> MSTSTVPPDGGEKVVVVGGNDWHEVVAAARAGAAAQAGERIVVNMGPQHPSTHGVLRLILEIEGEIITEARCGIGYLHTGIEKNLEYRNWTQGVTFVTRMDYL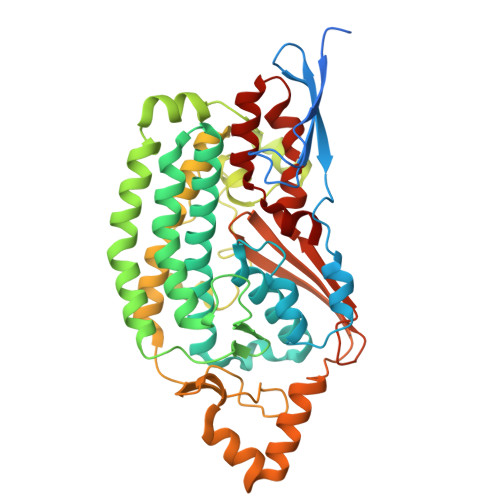SPFFNETAYCLGVEKLLGITDDIPERASVIRVMLMELNRISSHLVALATGGMELGAMSAMFYGFREREEILRVFESITGLRMNHAYIRPGGLAADLPDDAITQVRRLVEILPKRLKDLEDLLNENYIWKARTVGVGYLDLTGCMALGITGPILRSTGLPHDLRKAQPYCGYENYEFDVITDDRCDSYGRYIIRVKEMHESVKIVEQCLARLKPGPVMISDKKLAWPADLKLGPDGLGNSPEHIAKIMGRSMEGLIHHFKLVTEGIRVPPGQVYVAVESPRGELGVHMVSDGGTRPYRVHYRDPSFTNLQAVAATCEGGMVADAIAAVASIDPVMGGVDR> XSLSSKDKDTVKALWGKIADKAEEIGSDALSRMLAVY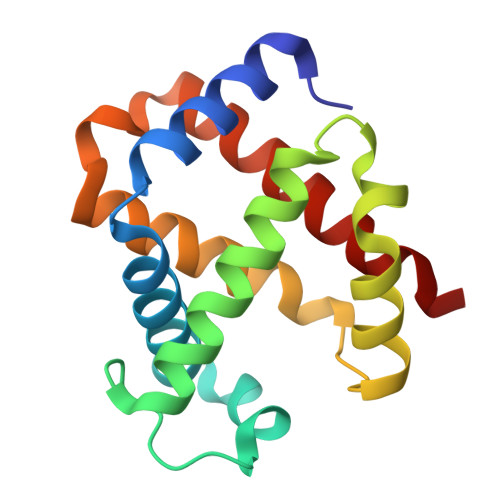PQTKTYFSHWKDLSPGSAPVNKHGKTIMGGIVDAVASIDDLNAGLLALSELHAFTLRVDPANFKILSHCILVLLAVKFPKDFTPEVHISYDKFFSALARALAEKYR>MSYYHHHHHHLESTSLYKKAGLENLYFQGMATPPKRSSPSFSASSEGTRIKKISIEGNIAAGKSTFVNILKQLSEDWEVVPEPVARWSNVQSTQDEFEELTMSQKNGGNVLQMMYEKPERWSFTFQTYACLSRIRAQLASLNGKLKDAEKPVLFFERSVYSDRYIFASNLYESECMNETEWTIYQDWHDWMNNQFGQSLELDGIIYLQATPETCLHRIYLRGRNEEQGIPLEYLEKLHYKHESWLLHRTLKTNFDYLQEVPILTLD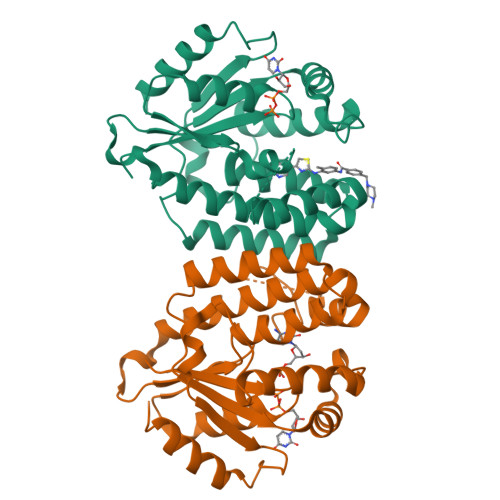VNEDFKDKYESLVEKVKEFLSTL[4x]>[4x]MALLTPDDLININMQLQKADSAVQEVTGLDIKGICKALYGTFSSSEKVGIVPVTSGNGIIGNFSASLHAITQYFGFDSFVTDMPDVSGYYEAVQNGAEIILMADDRTFLAHNLKNGKMA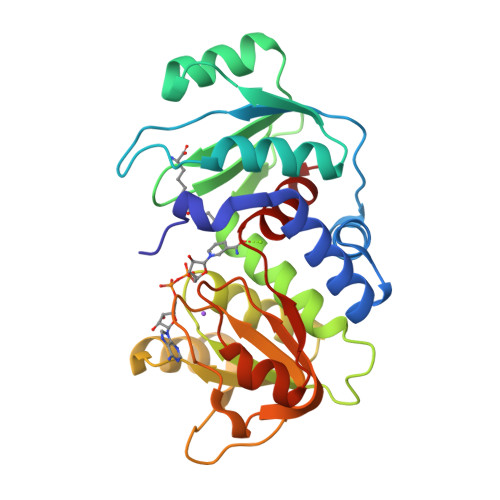NNQPCTGIIYAEIASRYLKADSKDVLVVGLGKVGFPGAEHLVQKDFRVYGYDADETLLERATSNLGIIPFDPANPKKFSIIFEATPCANTIPEAVLSENCVLSTPGIPCAISEELRDKYEVQLIAEPLGIGTASMLYSVL>GGGGRSVDTMALWLGLRAVLVVAGLAVLLQLIRGWLSSKSYVFNREEIARLAKEHSGLDYEVAFSKIIVELRKKHPGHILQDEDLQWVFVNAGGWMGSMCLLHASLTEYVLLFGTAVDTGGHSGRYWAEISDTILSGTFRQWKEGTTKSEIFYPGDTIVHEVGEATSVQW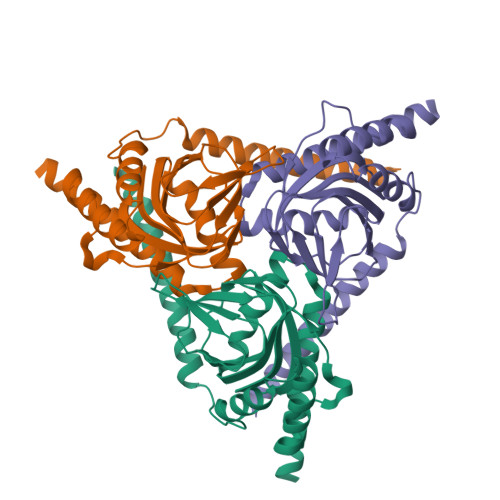SSGTWMVEYGRGFIPSTLAFALADTIFSTQDFLTLFYTVKVYSKALLLEASTHLSQLGFFAAA[6x]> DNGGYVPAVVIGTGYGAAVSALRLGEAGVQTLMLEMGQLWNQPGPDGNIFCGMLNPDKRSSWFKNRTEAPLGSFLWLDVVNRNIDPYAGVLDRVNYDQMSVYVGRGVGGGSLVNGGMAVEPKRSYFEEILPRVDSSEMYDRYFPRANSMLRVNHIDTKWFEDTEWYKFARVSREQAGKAGLGTVFVPNVYDFGYMQREAAGEVPKSALATEVIYGNNHGKQSLDKTYLAAALGTGKVTIQTLHQVKTIRQTKDGGYALTVEQKDTDGKLLATKEISCRYLFLGAGSLGSTELLVRARDTGTLPNLNSEVGAGWGPNGNIMTARANHMWNPTGAHQSSIPALGIDAWDNSDSSVFAEIAPMPAGLETWVSLYLAITKNPQRGTFVYDAATDRAKLNWTRDQNAPAVNAAKALFDRINKANGTIYRYDLFGTQLKAFAD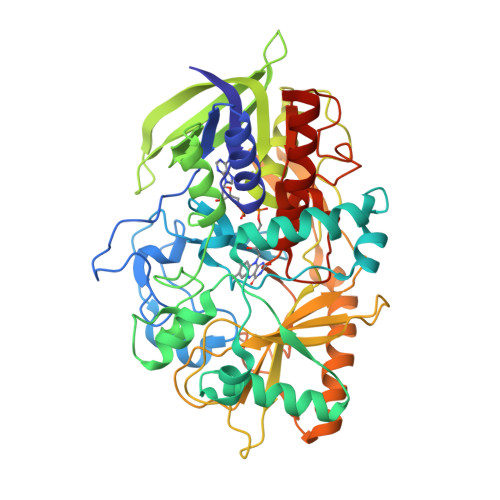DFCYHPLGGCVLGKATDDYGRVAGYKNLYVTDGSLIPGSVGVNPFVTITALAERNVERIIKQDVTASHHHHHH>MATGTWNEKERKEIPGFYNRFKTQAEKSTNTGLKGRLAMPIRANWGDVGKVVTIKNDLRQLKNLFGDDMNYSAFKLGKLALLGNVKELLLYRLVDGNQKKGTLTLKDTTENSAKDVIKLETKYPTARNFNVTIKSNLVDSDKKDFIFFENTKQLFSSSIKGTIDEIVLEINSNLDNEYVIATKVADSDTILANVVNQALEGGNDGCTSITNESYLKALEEFERYSFDSFVLDGVADEALQETTKAWVAKNKELGKDILLFLGG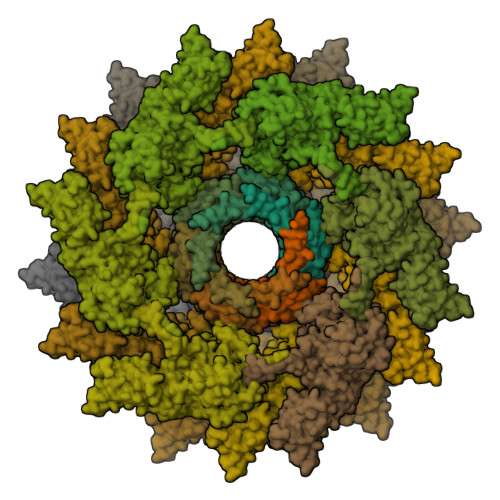KTEDNIKQINDKSKSFNDENIVNVGSSAYYENIKYTPSEVAVYIAALSVSKGITGSICNAKTIFEEVEPRLSQSEVKECLKSGTLVLDFDDGDVIIVDDVNTFKKYVDDKNEAMGYISNIMFINTINKDTSLKRKEFVGKIFNDATGQTTVICALKKYFEELMSQGIISEFNVDIDTELQATAKADEFYWKWDAVKVDVMKKIYGTGYLG[18x];>[18x]MYNDDYIEEASFLNGSDVVILIDGVEELYMEEIKADFEQDEQSIKLLGCQNEISRVGTTKGSFSLNGYKTDSKFAKLGFRSFEIIYNLSNSETLGYESIRLKNCRLKKLPLINSKAGEIVKIEVEGSFRGYDLLNEL>[2x]MEELDVDPAETPIPGLGQQNRHIGFSWGPGDLLLYETLYQKQGNSETAARCPFMYLVRSDEDIYSPVLRKLFNESHSIFVGLQKSAEEASGKSRKAQLVQVSRNYRSVLRACMEEMHTLSESTRETAQKYISQISILSAMELSWNLCEILFIESAPAGPLLILLLEWVRLHVCEVDNIVQDVLRSEKPTEHEKFWDGVTGYVLQGRMNEARQLLAKEASTSASARSMCRVLDDLLKKMPMLHTGGTQTLTEFELKWQHWREECERHLQNGTFSSNVHMEAVCRVLLGDEEVLLEKRDLMTTWYHFLVSRLLFKHPTVKPTELHFYAQSSLDMFLAGDSCPEPLDNILLAAFEFDIHQVIKEFSIVSSNWWFVAHLTDLLDHCQLFQAHNLYFGANMREFLLLDYASGLFSHHSLWQLGVDYFDYCPNLGREYLKLHMERIPLSTEKKALKALRICEQRQMTEQVRSICKTMAMQSLCNRRLGSALSWSIRAKDAAFATLISDRFLKEYCERGNFTDLDLIDNLGSAMLLSDRLTFLGKYREFHRMYSQEQFSEAASLLLSLMTARIAPCSFWLTLLLDALPLLEQKQVIFSAEQTYELMRCLEDRMAAKLESTSPDEIQKQDSSIDNTKVEMLRLALARNLARAIVTEGALQE;>[2x]MADKFAAKFVSHKISRTRWRPVSASSLQQPDVFATGSWDNEENKVCVWATSDFGATSLDEEYQGDPKQLCDIKHPGDVMDMQFLDKERIVTGSSTGTVTIFRHHENNQTLSVNQRWEQAHYHVGSNMRAPCTAIVCSSPEIVSVGEDGRINCFRAESRDVLRTIDDADSSTMHGVTFLRTTEILTVNSVGQLKLWDLRKQGNDPTQIFSVTGERVPLHCVDRHPNQQHVVATGGQDGMLCIWDVRHGKMPMSLLNAHEAEMWEVHFHPSNPDHLFTCSEDGSLWHWDASADSEKPTFLLGGRSTFNISRSSIAPPNANQSLACAWLSTDPTKGQLEITNLLPSSTLSVNSLDVLGQNLVCGTDAEAIYVTRRLFS;>MFVARSIAADHKDLIHDVSFDFHGRRMATCSSDQSVKVWDKSENGNWHCTASWKTHSGSVWRVTWAHPEFGQVLASCSFDRTAAVWEEIVGESNDKLRGQSHWVKRTTLVDSRTSVTDVKFAPKHMGLMLATCSADGVVRIYEAPDVMNLSQWSLQHEISCKLSCSCISWNPSSSRAHSPMIAVGSDDSSPNIMGKVQIYEYNENTRKYAKAETLMSVSDPVHDIAFAPNLGRSFHILAVATKDVRIFTMKPLRKELSSSGGVTKFEIHTVAQFDNHNSQVWRVSWNITGTVLASSGDDGTVRLWKANYMDNWKCIGVLKGDGNPVGNSYQGFFGSSVGSAGQSLQNSVNGTPSSGRKHS[2x];>[2x]MAAAESHMTSFQAEDWAGSNILPMVQRAGGSTRGIMAASVNLERSYMELIGAERETSRRNFRDLSLRPDVSLVIGGPKYSDCAGGYCYNESGSLLSATRNRFIHWTSYADTLELVELSLDINLLNNAVRLKILNCSILPGGVHICETQNNIIVLILTNQTVHRLILPHPSRMYRSEIISDSHIQSIFTDIGKTNFHDPNNTYVIPAIPGRAPNSTASTAWLSSDGEALFALPSVSGGILVIKMPPRDMEGLVTIAELKQSSVMQRLLTGWMPSSIRGDPGPAHLPVSLAVHTLDHDSYLFALCQDHKLRMWSYKDQMCLMVADMLEYVPVSKDIRQTAGTGHKLRLAYSDTLEILYLGVYLHTPRQGQFCVFQLVCTESNRYSLEHTSSIFTNQETLIDFTFTLSSMNIWALWLDDDNQTVMKHINFERNQAGHWNPVFVNPLPDDDLAIGDEQEPQEAYLECLFAPGRFTIAALQKAIQILRKGSGRVLDLSWEELKKEVTLTVEKEIQNAVVDYDVSQEEFRQINIENWCKFYTCCLQYQETLSRPLALVVHPNTNMVCLLRKGFLSFLAPCSSVEHLYLVPGEHLLTVDESVICDDVDGASDIVSLIQCLHMIADYITEDMAYQMESACCHPQSPERVAEQILEDLIANDIDNIMENIQNKLQDIRNPIQAISFLLQNMDYETNMDMEQSQHNVRLNLSTLYGSVTASSVVCQAIYKISATRFLICRDLLILQHLLLRLGDMALVGAGQLLHSQQELIPRAAQLLLSYYMIRWGSQCLACAVPVDLLESNLQHLSVLELSDSQVEKRRYTSGIQTIVELFFEDVGRKHFPQVFAHLFIQSGSSQVHRSLNWADLIHRITSYLLQLLWPSNPNFQFAECLMRNCQYTQLQEYVRLLLPWCQVNVGSCHFMLAQCYLVAGEGHKALDCFSQAASEVEREDFLEKLIRVEEGESVSPRLQYYNRVLRLLEDVGLPELVIQLATIAISEASDDWRSQAALRTRIFKHHLDMGHNSQAYDALTQIPDTSRQLDCLRQLVVVLCERSQLQDLVEFPYVNLHNEVVGIIESRARAVDLMTHNYYELLYAFHIYRHNYRKAGTVMFEYGMRLGREVRTLRGLQKQVNSYLACLNCLRLIRPEYAWIVQPVSGAVYERPGASPKRNYDGESSAVPSSSQIEILELRDLEKEYVLAQTRLTLAKHNPSTAAIAGSSAAEEMVALLVQAGLFDTAISLCQTFKLGLTSIFEGLACKCIRLQQGGEAAQAEAWEWLAANQLATVITTKESSATDEAWRLMISYLDKYESKNTLYHHCIINKLLSHGVPLPNWLINRYKAMDAAELLRLYLKYDLLEEAAELVLEYVDALLGKGHQYFGIQAPLSATSQLVWFPYSAIDHLRLALGENENNQHNQAILGKLQRKMDEYFQKLKKATDDYKKIVQKPVRA;>[2x]MKQDSASNATYTVDCEDYVHVVEFNPFDSGEAGSLLAYGGISYVVIASCRFQEEDSTVEGIEFKTLKTFHHGERVVAIAWSPETRCDALLPLLRFATAAGDKKIRIFTSDFQDKNEYKVIEGHSGYINDLVFCSPEGTDIASVGDDHTCRIWDLDGKQIAMFILRSPGMSVAWHPEGAFKLMVAEKTGTIRFYDLTTHQAILSLESVQVPLMSADWCVRNTLRIGAVAGNDWIIWEMPRSSYPQDNKPAHADRARMFRWSKCNENVFATTGYPGKMKSQIAIHHLAHPQPILIGTAPVGSGLSWHRRLPLCVVGGYRKLFFWLTEM;>SKYGLQDSDEEDDQLNSAEAKKLKTAPVPPQGKQPPLQQATLPGKVTPPPQSPAVDQLDRVMELDSDMADITQDQDLDSVAEEQDISEEQEPLSASSHIASSLGINPHALQVMKASLLLEEEDGEIMSRFSSFPSSMDPYPDVRSPRLFPSSHAKRPSSIGLLQSKFSAPSMSRLSETVQGSHSPKIHPAAPWSVPAPLAPSFIMPGPAPDTHLRTVGTRRQQELVPLEKSVTHGRGTLMIDMGLFMGRSFRVGWGPNWTLVHNGDKLSERLNAEEDRDMDTIDYGFLPKPTSAKSLTESPFKVHVEKLSLEQKTKDLQSYLLPLEIELKNSTVDKSGPCPHFRPNPGVTAIHDYAGWVRNFSSEAAEVEAVVKQWGLTWTLCESLWGQLKELEASLDEPNEYVKNLERRKAFSHWLAQTAQERIEEEVSLYGPERHIEAVFSYLTGGRISDACRLAQKSGDHRLSLLLSQMVGSQEVRDLITLQLVDWNKLQVDHYIQEERLRVFCLLSGTPVWRSSDNRSINVCSQLDWKRTLGIHLWYMLPPTATVAQALHMYEQAFQEQEGGEPYACYPLPPYLEDCGFSFGDDPSAKFISLQRDVCVHLLKLYSERQYDLCQLLDPSSATPDPLDYRLSWHMWMVLQALNYTHLSGHRQGMLHASYAAQLENVGLWEWAIFVLLHIQDPHVREAAVRELLNRHCVVHDSPESLAKENFLIQRLCLPAQWIHKAKAVRSRRDGDKHKEALYLLKSHQWNQCHKLVTRHLAADAVINENYRYLRGFLGELARPEHCKHIQDWETAGKVYLDYISVIEMLNQIRQDECSGGELEKLHTKVMSLCKWVELIQCYSAKGRLAQSEMAKRVANILRVVLSLQQPPESMSDSSSEPRVPLRLLAPHIGRLPMPEDYALEELRGLTQSYLRELICGS[2x];>[2x]MVSVINTVDTSHEDMIHDAQMDYYGIRLATCSSDRSVKIFDVKNGGQILIADLRGHDGPVWQVAWAHPMYGNILASCSYDRKVIIWKEENGTWEKTYEYTGHDSSVNSVCWAPHDFGLVLACGSSDGAISILTFTGDGPWEVKKISNAHTIGCNAVSWAPSVIPGSLVDQPSSQKPNYIKRFVSGGCDNLVKIWREEDGQWKEDQKLEAHSDWVRDVAWAPSIGLPTSTIASCSQDGRVYIWTSDDAATNCWTPKLLHKFNDVVWHVSWSITANILAVSGGDNKVTLWKESVDGQWACISDVNKGQGAVSTVTEGQLNDQ;>[2x]MDMLSPVVREAEVSRAARRQSSNRKNPADESWSNATPTRGPSSRTTGQTLFRQHMTPQTWNSSRPPDVSAILGTVGRSPRLLQTPGRLANLSMMSNPDDSVWTTTFSPGRTGMYTTLDSPSFTEDITLSAVMLQEEDPGEAATMSMYPDFLKSFLEHPSSAVFELIEQYEATCNTQITLLKKIVKRVTPGQQKFSKTASILWLLQQEMVTWRLIAALYRDRIQSALEEENMFEIAAPNASEKTIVDKLFQRDTLVRQSQLVVDWLESIAKDEVGDFSDNIEYYAKSVYWENTLHTLKQRSMLSLGSSRPLVSELDPDAPIRQKLPLDDLDREDDIRLLKYLFTLIRAGMTDEAQRLCKRCGQAWRAATLEGWKLYHDANINGGTELQAVEGNPYRCVWKTCCWRMAEDEQFNKYERAIYATLSGNLKQLLPVCESWEDTVWAHFKVMVDSLVEQEIRASIISFNEANELPREYLEANWTLDSVFEELQATDKKRVLEENREHYHIIQKFVILADVDGLMDEFSEWLSNGKNLLLGHLLRFMTHLLLFFRTLGLQAKEEVSVEVLKTYIQRLINEKQIELIAFYVSHLPQELAISQYAVFLENITDPDQRQRCLELAKEAGLDVASITKTVVENTRKKDAGEFAHHDFAPALDSGTSEEDRAKIDVIDWLVFDPAQRAEALKQSNAIMRKFLASKKHEAAKEVFAKIPQDSIAEIYSQWEEQAMDSALPAEDDNAIREHLCIRAYLESHEAFNEWFKHINSPPQKPTLVGQASFTEKVAHEHKEKKYEMDFGIWKGHLDALTSDVKEKIYNVLLFVDGGWMVDVREDTEEDPERSHQMVLLRRLCLPMMCFLLHTVLHNTKQYKDCLRLADIVSSENQKLYTVFSKTEMRNLLQKLRESSLMLLDLQLDPLGYEIQS;>MFPSPRAQGMGSARRPFNSRLTGGRKALGPGVTASSSPSALYSPVGRRVSASGARSTPSRVYLHPAASETVNYNVQLFGSSLPVKVMEALSNASADEPMAACIHEGGWAWLACNDRLIIWKISHSSSAKLMVCKELPLPLSDSEWSADLVDICAQTGDPAAAQSVALMAATPEGSSRYWPNILHEGTYIESYTEFGSSLCAFVTAVKGNSFILSSEKNQLVRLTPDASGKMNQRVLPQGQGMLSGIGRRVSTLFGILSPAVESTLCSVLWDKGDCFYTLTDSSINKWDLDDTSESQVLNWDMSRVLREYISDAIWGSESDYDDIKAGININYLSLNQNCDGLVILSAAWHPGDNPCQIYYTLVTVKDEGYNISDEITVEVTQFNPVFQARGMQLCQLVVPNFSSQACYLYTQEMIFACSTGTGRSTLPQEKIPFEAQGDNIVGAGSCEGWPVFFIRKSGMLTVVARETASVLPEHMEESLSSVSKSSRQAVVKDSRPDQIAHDDKTKHLKAAFLRYCRKDILGAQSMVDSLFSDSDMEPDDELDLAVNQISVDLIDDYPASDPRWAESVPEEAAGFSNTSLILLHQLEDKMKAHSFFVDFLHQVGLFSRLSTCQTKGMLVATRLLLSEHAEKLSAAIVLKNHHAKLPVLVNSAIQLALDKRMCTVPQNLTAADVYFREVSQMEIIFECLVDKEEADLESTSIDSVEWANIVVNVNTILKDMLHVACQYRQSKNSLYKNESGIQEPEHVPWTASSGTAGIRSVVTRQHGIILKVYPQADSGLRTILIEQLAALLNYLLDDYVTQLKSIDKLANEERYNILEMEYAQKRSELLSPLLILGQYAWASNLAEKYCDFDILVQICEMTDNQSRLQRYMTLFAEQNFSDFLFRWYLEKGKRGKLLSQPASQHGQLAAFLQAHDHLSWLHELNSQEFEKAHRTLQTLANMETRYFCKKKTLLGLSKLAALASDFQEDVLQEKVEEIAEQEHFLLHQETLPKKLLEEKQLDLNAMPVLAPFQLIQLYVCEENKRANENDFMKALDLLEYIGDDSEVDVEELKLEILCKAIKRDEWSATDGKDDPIEATKDSIFVKVLQNLLNKGIELKGYLPKAETLLQSEELNSLKTNSYFEFSLKANYECYMKMQS[2x];> MAAQLALNSEASLWGPYREIWQTVLSALIKRQPEAVHSLDIVLKKYKPDFISLFKNPPKSAQQHERVQKASTEGIPIKGTQRTRILEEQLIKEAFILSDLYNIGEIAAVELLLIGEQQQPTFHGLTRGLVAILLYWDGKSCMAESLLHLIQARKGKTFTLDHSPEVVSMVTRFTDDLMEQGLTNKILTLISQIDVNNEFDKLKKERGLGNKKHRKEVSDLIKECQQSLAHSLYSWSCQTPLNREDTLLLIGYLEKVTVEGDGSLDKVNLTLLMSLLYCLDVGFLEQGTDDREELMKQASMFMDRQYIAAIHNRLQNTQPWKSPGMQATVRLAWALALRGISQFSEVLEFSEADEPMAEIAIGGNVFLFLTEAVVGSESFCTDEFFIRRIHKLVTDFPTLMPMKVKQLRNRAEEDARLIQMSMQMGNEPPASLRRDLEHLLLLIGELYRKDPFHLELALEYWCPTEPLQSTSLMGSFLGVAHQRPPQRQVLLSKFVRQMSDLLPATLYLPYLKMLRGLASGPQCAHYCFSLLKANGGSSAENLQAAGGSPVSWDHFFHSLMLYHEHLRRDLPNTDNIHQRHPPLRGITQRELDGLIACLQLTCTIIDWSESARLALCEHAQWMPVVVILGLLQCSIPPLLKAELLKTLAAFGKSPEIAASLWQSLEYTQILQTVRATGLRQGVGIEVELNEIESRCEEYPLTRAFCQLISTLVESSFPTNLGAGLRAPGFEPYLQFLRDTVFLRYRTRAYRRAAEKWEVAEAVLDVFYKLLKDYEPQPEDFVDQYVELQGEERVAFKPPGFSLMHHLLNESPMLELCLSLMEEGVTQLDTYAPFPGKKHLEKAVAYCFMLLNLTLQKENRFMDLLRESHLSMIVTPLEQLLQGINPRSKKADNVVNIARYLCHGNSNAELAFESAKILCSISCNSKIQEKIVGDFTQDQNVSQKLMVGFVSCLDSEEAEELLDSEKEAEDQVKQTNIRYMTKIHILNLLITSLEMKAPNLAMFLLGYELKKPVSTTNLQDSGVLGCPRTCLHSILDILRKGTDVRAGPVAVWDTPHLAELCYQVIYQLCACADTSGPTMRYLRTSQDFLFSQLQHLPFSVEESEISAMNQMSWLMKTATIELRITSLNRQRSHTQRLLHLLLDDMPTRPYSADGEGGMEDESRSLSGFLHFDTTSKVRRKILRILDSIQFSNEIPEPLQLDFFDRSQIEQVIANCEHKNRRGQTVCNVKLLHRVLVAEVNALQGMAAIGQRPLLMEEINTILQYVVERNKLLQCLHAKRHALESWRQLVEIILTACPQDLIPTEHRQLIIRDLLQDLHVKILDDDAAQELMPIVAGAVFTLTAHLSQSVRTELKQPMTASGLGQSQYVQMLDGSFAAPPGTENISAGFASIGDSSLHMILRNLLEFILKTGGGFQRVRAHLYGSLLYYLQIAQRPDEPDTLESAHKSMWERLTAPEDVFSKLQRDNLSIFESYGTALMEVVCRDACDGHDIGRMLALALLDRIVSVDRQQQWLLYLSNSGYLKVLVDSLAEDDVVLRNLLTPQPPLLKALYIYESKMAFLTRVAKSSQGAIELLRSGVIVRLAQCQVYDMRPETDPHGVFGMRETPVFIPAPVERYRQILLPALQICQLILTSSTAQHLQAAGQVLQFLVAHSDTIQAILRSQEGSLGSLQELALLTGIISKAALPGVLNELDIGLNDGSMMELQGHIGRFQRQCLALLNRFGGSDRLRQLSLQDDSSRLDGVSKKDDMELAMQQICSNVMEYCQALMIQNSPSFQQTVCLFTPSLKESASRDGTRQDSQVSILPSWRLPSLGVVIHLLKQSANNFFTYYDIHRQSVGKLQNVEQLPPDEIKELCQSEMPVGADKISTTQKYGLARRRLVKLINSRAKLLSLCSYIIETCLYILWRHLEYYLLHCTTSDSQDPVFSNMTFGNRRFQDTFNTDPNMDPRNLRQNKVSQQDVDTLLREGANSFGESLQKRLLDIESLYCKVRSRHSFIQALVRRIRGLLRVSRV;> MQNLEAQVTGSLVAFPDVTQKALKEDEINLDSVLRGKFSTGRTSLAWLACGPQLEITNSVTGERISAYHFSGLTERPPVVVAVKEFTWQKKTGLLVGLVEAEGSVLCLYDIGISKVVKAVVLPGSVTAVEPIINHGGASASTQHLHQSLRWFFGVTAVVTDVGHVLLIDLCLDEVSSNQDELDASDLEVMSVIPTKIPKLREAATRERRHLCLQLAAPTGTTVSCLSYISRTNQLAVGYSDGYFSLWNMKTLRRDYHVQIEGGRVPVCAVAFQEPENDPRNCCYLWAVQSSESGGDVSLHLLQLAFSDRKCLASGQIMYELLEYCEERYSLDLSGSTLSLRGQSNNTKLLGCQTIEKFRVHGEREDGVHEVTSPDTSVSVFSWQVNTYGQGKPSVYLGVFDINRWYQAQMPDSLRSGQFLRNCSYFAFWSLEAVVNITTQDIIFDILVHERSLSRGIPPSYPPPEQFYYPSTYNFDATCLLNSGLIHFACTGFQKETLHFLKKSGSSLNEAIPDGYNRCLAAGLLAPKFTDVQASSLSQEEQLQAILAAAVETSSLGLLTSCIKRWTAEEQPRSAANLRFVLEWTWKKVTLTKQEFDRLCFRLFDGSCNFIDPHTLQSLQQCHLYFSNLTAVLNCFIAQAKEVTQQGAVDLTNKQSVTRLLTLYASVVLWFCRSGMLPDSSDETVQLTRPFYNYQVIQQYYSDQRKKLERLARGKWDTSSLMIDGLINQFGDRIQQLWSRDDNGTGKYPPANLHALLDVYLLENADEMSKHAITIYFLLDIMYSFPDKPDSSIESFPTAFFVPGSLIKLIQGFWLLDHNDYQNSVDCILNPASSRVMSWQHSQIIENLLCHGDSRQALRYLQVMKPVATTSKEVKLHMTVLLANRSILEAWNLQRLHSSRLNVEELLKHMYEMCQEMGLIEELLKLTFTDFEQGYLHKFLQTTGVQNQELLLVHHLQRANYISALQLNQSLKTNHLNDCDRRLRERSGARNAILDQYGKILPRVQRTLASERAKPYSLPSLVWREVARPKPLSTTAKQAAPGSIITKANFICNVLSKIKEVSTANEKREEYSPYQSMVSEEPTAPPLQDIDVPDAFFGTPINKSRRVSRLLDSVVHPVLMEPTPLTSSDTDNNQTPHKSPLLKTSSPLHSSLRRIAHMRSFAKASEFSLLETPLVVRKAKALAANTASSGYTSITPQSILRSSVRTTPLVSPSVSPGRSLTPPLRPKETKISFMELSFTRHAKAAHSSEGNLLAISPVLRSSPDAVWSVKGKVASFTQNTPVKKLDEIDASSSGIQEESQDEMEVSKEISNISVRSEQASLEYHDAPTPEDLENDEISGTTNSQPQVNEVHHQMEDGQLTEKPAELALTEMQEEFIDSEEREIEYISAPLNGPNALECMTAVPDIYLEDASQCILETPEGSSVSVTGEQECVSSAKDSESVISIHDSDDAHSNLSENDQDSEEIEENNLRVPTTVTRCEEFDLIETKDLEVELEEADSEKTNYKDIYPDATVQLGFTVESIEQRYTCELADRRETPSETDEIEGEHFETENNFSLVLEGDVTEEEILEPSSSKTDLELTRPPIAHQKLISENRENIENCETTEKIPANMSPLVDSDHESKTLETLPSEADLSVAEKVLKGTEEKDVPPEVHSEVVLESKLVGNAMMSLDSSESQEVIISQYDNVISIEKLEMTQEKMYGEKTEQINEGQVSPNRDQSTLVKPLTPRRSIRKSSKPADSSTDIIGNITLPTTPKRGLKKAKENVDTLKNSISVVPEEELTLGTRRITRKATLTALDNPEPLQIKEPPSGEDLQVQPSTPTRGRRGKVITSDDLKEPPSGEDLQVQPSTPTRGRRGRVITSDDLREPPPGEDLQVQPSTPTRGRRGRVITSDDIKESPSVEDLQVQPSTPTRGRRGKVITSDDIKEPPSVEDLQVQPSTPTRGRKGKVITSDDIKEPLSGEDLQVQPSTPTRGRKGKVITSDDIKEPLSEEVLQEQPSTPTRGRRGRVITSDGKGYECVEEKNALPLTPTRITRSKNILEPEKGISQIEPEKGISQIEPDKGLSQIEDTGETEHEVVTPRRGRRGKRVVNELVKHFERNSSQPNIKADTSPPVSPKKVSLRWTRTRSENQRINATEEQASKIQEDLSDTPRKRYKKSSNKMGFEETTDTVTEGAIVEDVQESLIISHLGKNPNTSIVRSARKTALPPVTEDHSEQPLLPPESHSKVHSSLAIADEENKTNTRTRSGNKSSVDVSAITFEFSTPKARTKKTAKGSAVPTELIPSTQYVFSPPSTRTRRATRANVSEAVIEPQLQFQESCEIAETEVPEVPASKPRGRPPKHKAKAVTRVLKKPSWSTPPVEIKLISPPESPAVSETNTKTDSTEAKGAEKISVRRTRRRIIAKPVTRRKMR;> MDGEGFGELLQQAEQLAAETEGVTELPHVERNLQEIQQAGERLRSKTMTRTSQESANVKASVLLGSRGLDISHISQRLESLSAATTFEPLEPVKDTDIQGFLKNEKDNALLSAIEESRKRTFVMAEEYHRESMLVEWEQVKQRVLHTLLASGEDALDFTQESETSYISESGAPGRSSLDNVEMAYARQMYMYNEKVVSGHLQPSLVDLCTEAAERLDDKNVSDLWVMVKQMTDVPLIPASDTLKSRCSGQMQMAFVRQALNYLEQSYKNYTLISVFANLQQAQLGGVPGTYNLVRSFLNIRLPTPIPGLQDGEIEGYPVWALIYYCMRCGDLMAAQQVVNRAQHQLGDFKNCFQEYIHNKDRRLSPTTENKLRLHYRRAVRASTDPYKRAVYCIIGRCDVSDNHSEVADKTEDYLWLKLSQVCFEDEANSSPQDRLTLPQFQKQLFEDYGESHFAVNQQPYLYFQVLFLTAQFEAAIAFLFRLERTRCHAVHVALALFELKLLLKSTGQSAQLLSQEPGEPQGVRRLNFIRLLMLYTRKFEPTDPREALQYFYFLRNEKDNQGESMFLRCVSELVIESREFDMLLGKLEKDGSRKPGAIDKFTRDTKTIINKVASVAENKGLFEEAAKLYDLAKNPDKVLELTNKLLSPVVSQISAPQSNRERLKNMALAIAERYKSQGVSAEKSINSTFYLLLDLITFFDEYHAGHIDLSFDVIERLKLVPLSQDSVEERVAAFRNFSDEIRHNLSEILLATMNILFTQYKRLKGSGPTTLGRPQRVQEDKDSVLRSQARALITFAGMIPYRMSGDTNARLVQMEVLMN

The nuclear pore complex (NPC), one of the largest protein complexes in eukaryotes, serves as a physical gate to regulate nucleocytoplasmic transport. Three scaffold rings, including an inner ring (IR), a cytoplasmic ring (CR) and a nuclear ring (NR), anchored onto the nuclear envelope (NE), provide bases for other functional parts, such as the cytoplasmic filament, nuclear basket, and permeability barrier. In both CR and NR, named the outer rings, the backbones in each subunit are formed by one or two Y-shaped complexes, also known as the Nup84 complex in fungi or the Nup107-160 complex in vertebrates. Here, we determined the 8 Å resolution cryo-electron microscopic (cryo-EM) structure of the outer rings containing nuclear ring (NR) and cytoplasmic ring (CR) from the Xenopus laevis NPC, with local resolutions reaching 4.9 Å.

For NR, the final average resolutions were 8.1 Å for the NR subunit region, 7.8 Å for the NR core region and 8.6 Å for the NR Nup133 region, where the highest local resolution reached was 4.9 Å for the most rigid part of the NR subunit. In our model of NR, a total of 15664 residues were built in each subunit, so we extended the number of residues by approximately 82.6% compared with the NR of the 2015-model (8,578 residues) and by approximately 41.6% compared with the NR of the 2016-model (11,064 residues). However, in this study, according to the high-resolution and isotropic cryo-EM map of the X. laevis NR, we found only one copy of the ELYS density situated on the convex side of the inner Nup160 in each NR asymmetric unit. The AlphaFold2 predicted model of the ELYS NTD is fitted well into our cryo-EM map of NR. It is obvious that ELYS has extensive and tight interactions in both the β-propeller domain and α-solenoid domain with the inner Nup160 (β-propeller domain and α7-α34), suggesting that during the ELYS-mediated NPC assembly process, Nup160 could be easily recruited by ELYS. The 9th to 12th α-helices (S555-G675) of ELYS come close to the 8th α-helix (D557-N578) of the inner Nup133 in the adjacent NR subunit, stabilizing the head-to-tail connection of the NR subunits. Therefore, it can be concluded that the question mark-shaped density represents Nup205 not Nup188 in the NR subunit of X. laevis NPCs. In the MID, the tower helix of Nup205 (α55-α57, E1195-T1293), together with the finger helix of Nup107 (α34, Q770-F814) in the adjacent NR subunit, is inserted into the grooves formed by Nup85 (α23-α25, D493-E549) and Nup160 (α40, G1255-S1282). In the CTD, the 63rd and 64th α-helices and 75th to 84th α-helices of Nup205 form tight contacts with the 1st to 4th α-helices and 7th and 8th α-helices of inner Nup107 in the adjacent NR subunit, respectively. These results suggest that Nup205 plays an important role in stabilizing the head-to-tail connection of asymmetric units of the NR.>[2x]GVSDESV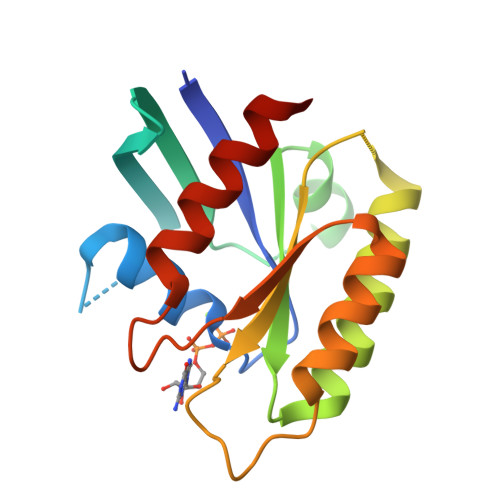YKVLLLGAPGVGKSALARIFGGVEDGPEAEAAGHTYDRSIVVDGEEASLMVYDIWEQDGGRWLPGHCMAMGDAYVIVYSVTDKGSFEKASELRVQLRRARQTDDVPIILVGNKSDLVRSREVSVDEGRACAVVFDCKFIETSAALHHNVQALFEGVVRQIRLRRDSK> GSSHHHHHHM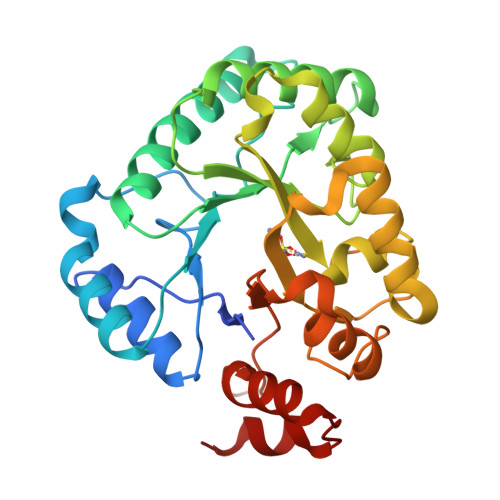LKIGSHVSMSGKKMLLAASEEAVSYGATTFMIYTGAPQNTRRKPIEELNIEAGRKHMEQNGIEEIIIHAPYIINVGNTTKPETFQLGVDFLRMEIERTSALGVAKQIVLHPGAHVGAGADAGIQQIIKGLNEVLTPDQTVNIALETMAGKGTECGRSFEEIAKIIDGVKYNEKLSVCFDTCHTHDAGYDIVNNFDGVLNEFDKIVGIDRLQVLHINDSKNVRGAGKDRHENIGFGHIGYKALHHIVHHPQLTHVPKILETPYVGEDKKDKKPPYKLEIEMLKNGTFDEGLLEKIKAQ> MSMYTTAQLLAANEQKFKFDPLFLRLFFRESYPFTTEKVYLSQIPGLVNMALYVSPIVSGEVIRSRGGSTSEFTPGYVKPKHEVNPQMTLRRLPDEDPQNLADPAYRRRRIIM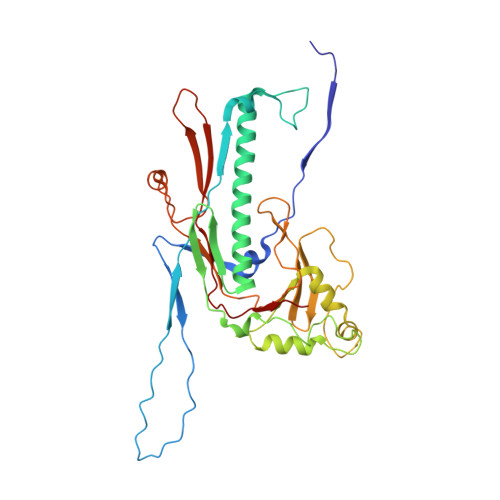QNMRDEELAIAQVEEMQAVSAVLKGKYTMTGEAFDPVEVDMGRSEENNITQSGGTEWSKRDKSTYDPTDDIEAYALNASGVVNIIVFDPKGWALFRSFKAVKEKLDTRRGSNSELETAVKDLGKAVSYKGMYGDVAIVVYSGQYVENGVKKNFLPDNTMVLGNTQARGLRTYGCIQDADAQREGINASARYPKNWVTTGDPAREFTMIQSAPLMLLADPDEFVSVQLA>SNAMKVINVDVAIIGTGTAGMGAYRAAKKHTDKVVLIEGGAYGTTCARVGCMPSKLLIAAADASYHASQTDLFGIQVDRISVNGKAVMKRIQTERDRFVGFVVESVESFDEQDKIRGFAKFLDEHTLQVDDHSQVIAKRIVIATGSRPNYPEFLAAAGSRLLTNDNLFELNDLPKSVAVFGPGVIGLELGQALSRLGVIVKVFGRSGSVANLQDEEMKRYAEKTFNEEFYFDAKARVISTIEKEDAVEVIYFDKSGQKTTESFQYVLAATGRKANVDKLGLENTSIELDKKNSPLFDELTLQTSVDHIFVAGDANNTLTLLHEAADDGKVAGTNAGAYPVIAQGQRRAPLSVVFTEPQVASVGLSLRQIEDLYADQDAANYVVGQVSFEGQGRSRVMGKNKGLLNVYADRTSGEFLGAEMFGPAAEHIGHL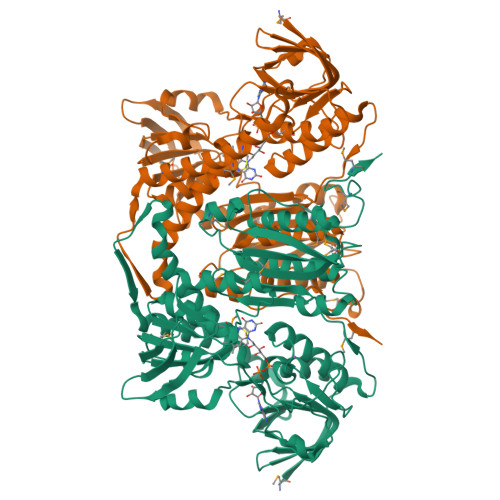LAWARQQQMTVQAMLTMPFYHPVIEEGLRTALRDAQQKLAIEKHDMNEFIMTHDNAMKLVI[4x]N-{4-[(3-phenylpropyl)carbamoyl]phenyl}-2H-isoindole-2-carboxamide 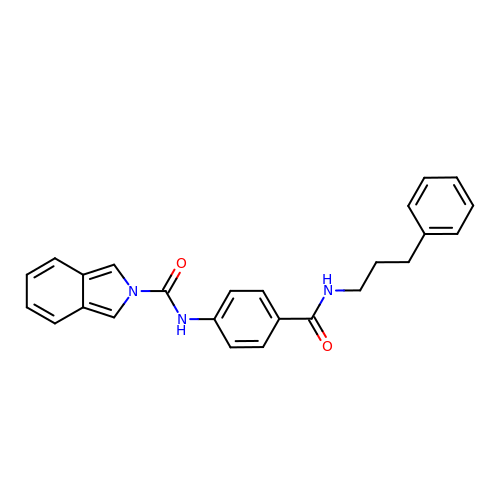| C25 H23 N3 O2 | YXCPDCLETYPTMF-UHFFFAOYSA-N4-[(trans-4-aminocyclohexyl)amino]-N-(6-chloro-3-{[(2,5-difluorophenyl)sulfonyl]amino}-2-fluorophenyl)thieno[3,2-d]pyrimidine-7-carboxamide 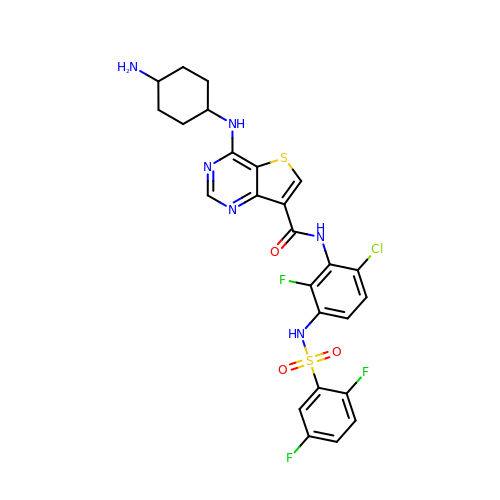| C25 H22 Cl F3 N6 O3 S2 | NALUYXQOXMHJMM-HDJSIYSDSA-N>MNLLVTSSLGVLLHLVVLCQADDHSELLVNTKSGKVMGTRVPVLSSHISAFLGIPFAEPPVGNMRFRRPEPKKPWSGVWNASTYPNNCQQYVDEQFPGFSGSEMWNPNREMSEDCLYLNIWVPSPRPKSTTVMVWIYGGGFYSGSSTLDVYNGKYLAYTEEVVLVSLSYRVGAFGFLALHGSQEAPGNVGLLDQRMALQWVHDNIQFFGGDPKTVTIFGESAGGASVGMHILSPGSRDLFRRAILQSGSPNCPWASVSVAEGRRRAVELGRNLNCNLNSDEELIHCLREKKPQELIDVEWNVLPFDSIFRFSFVPVIDGEFFPTSLESMLNSGNFKKTQILLGVNKDEGSFFLLYGAPGFSKDSESKISREDFMSGVKLSVPHANDLGLDAVTLQYTDWMDDNNGIKNRDGLDDIVGDHNVICPLMHFVNKYTKFGNGTYLYFFNH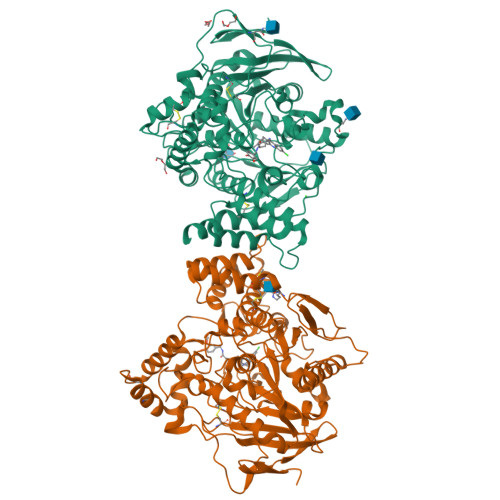RASNLVWPEWMGVIHGYEIEFVFGLPLVKELNYTAEEEALSRRIMHYWATFAKTGNPNEPHSQESKWPLFTTKEQKFIDLNTEPMKVHQRLRVQMCVFWNQFLPKLLNATACDGELSSSGTSSSKGIIFYVLFSILYLIF[2x]>[4x]QADFEHAISDLEAHNQAKIGVALVSENGNLIQGYRANERFAMCSTFKLPLAALVLSRIDAGEENPERKLHYDSAFLEEYA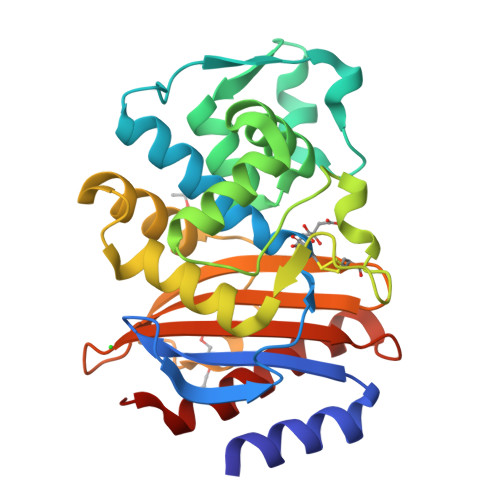PAAKRYVATGYMTVTEAIQSALQLSDNAAANLLLKEVGGPPLLTKYFRSLGDKVSRLDRIEPTLNTNTPGDERDTTTPMSMAQTVSKLIFGDTLTYKSKGQLRRLLIGNQTGDKTIRAGLPDSWVTGDKTGSCANGGRNDVAFFITTAGKKYVLSVYTNAPELQGEERALLIASVAKLARQYVVH>[2x]TGTSEMAPALVAAFGG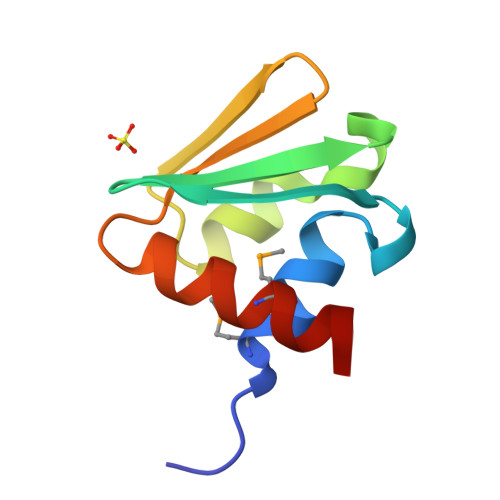KENITNLDACITRLRVSVADVSKVDQAGLKKLGAAGVVVAGSGVQAIFGTKSDNLKTEMDEYIRNH>[2x]SMSHYKSNVRDQVFNLFEVFGVDKVLGADKFSDLDADTAREMLTEIARLAEGPIAESFVEGDRNPPVFDPETHTVTLPEGFKKSMRALFDGGWDKVGLAEHLGGIPMPRALQWALIEHILGANPAAYMYAMGPGMSEIFYNNGTDEQKKWATIAAERGWGATMVLTEPDAGSDVGAGRTKAVQQPDGTWHIEGVKRFITSADSDDLFENIMHLVLARPEGAGPGTKGLSLFFVPKFHFDHETGEIGERNGVFVTNVEHKMGLKVSATCELSLGQHGIPAVGWLVGEVHNGIAQMFDVIEQARMMVGTKAIATLSTGYLNALEYAKERVQGADMTQMTDKTAPRVTITHHPDVRRSLMTQKAYAEGLRAIYLYTATFQDAEVAQAVHGVDGDLAARVNDLLLPIVKGFGSETAYAKLTESLQTLGGSGFLQDYPIEQYIRDSKIDSLYAGTTAIQAQDFFFRKIIRDKGQALAYVAGEIEQFIK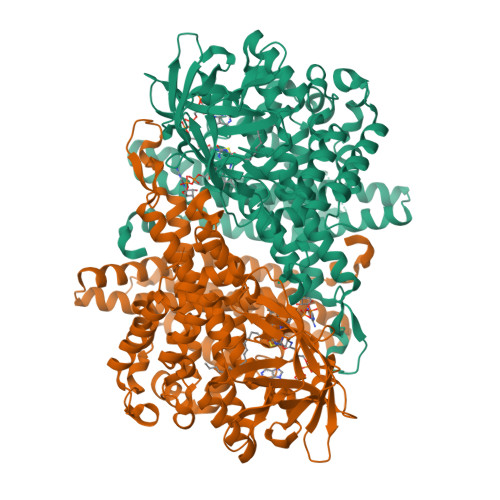NENGNGRLKTERELLATALADVQGMAASLTGYLMAAQEDAASIYKVGLGSVRFLMAVGDLLSGWLLARQAAVAIEKLDAGATGADKSFYEGKIAAASFFAKNMLPLLTSTRQIIENLDNDVMELDEAAF> GSGPPGPPGPPGPPGARGQAGVMGFPGPPGPPGPPG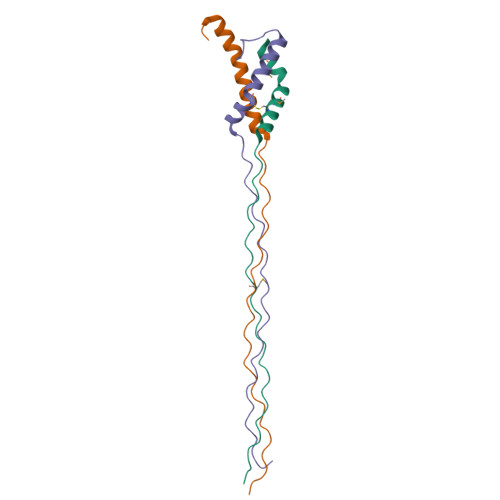RAPTDQHIKQVCMRVIQEHFAEMAASLKRPDSGAT;> GSGPPGPPGPPGPPGARGEPGNIGFPGPPGPPGPPGRDATDQHIVDVALKMLQEQLAEVAVSAKREALGAV;> GSGPPGPPGPPGPPGARGQAGVMGFPGPPGPPGPPGKEASEQRIRELCGGMISEQIAQLAAHLRKPLAPGSI>LKINQQEEPGFEVITRIDLGERPVVQRREPVSLEEWTKNIDSEGRI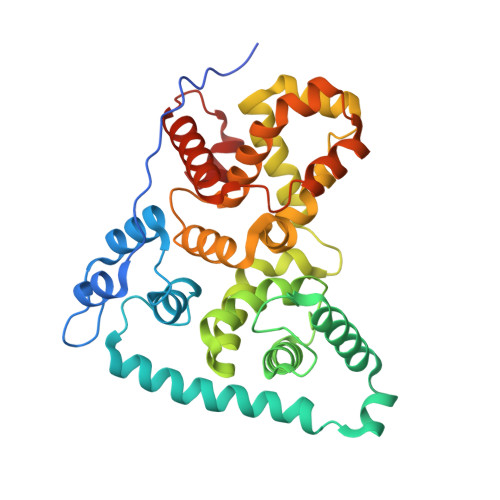LNVDNMKQMIFRGGLSHALRKQAWKFLLGYFPWDSTKEERTELQKQKTDEYFRMKLQWKSVSEEQEKRNSRLRDYRSLIEKDVNRTDRTNKFYEGQDNPGLILLHDILMTYCMYDFDLGYVQGMSDLLSPVLYVMENEVDAFWCFASYMDQMHQNFEEQMQGMKTQLIQLSTLLRLLDSGFCSYLESQDSGYLYFCFRWLLIRFKREFSFLDILRLWEVMWTELPCKNFHLLLCCAILESEKQQIMEKHYGFNEILKHINELSMKIDVEDVLCKAEAISLQMVKCKELPQAVCEILGLQDSE[2x]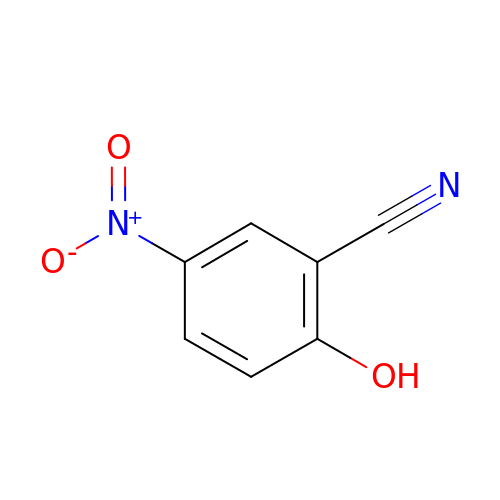5-nitro-2-oxidanyl-benzenecarbonitrile | C7 H4 N2 O3 | MPQNPFJBRPRBFF-UHFFFAOYSA-N> GSKPIDVFDFPDNSDVSSIGRLGENEKDEETYETFDPPLHST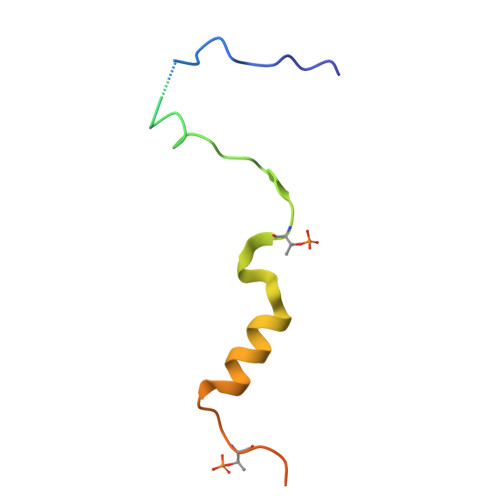AIYADEEEFSKHCGLSLSSTPPGKEAKRSSDTSGNE> SSVEKKPEGVNTGAGDRHNLKTEWPELVGKSVEEAKKVILQDKPEAQIIVLPVGTIVTMEYRIDRVRLFVDKLDNIAEVPRV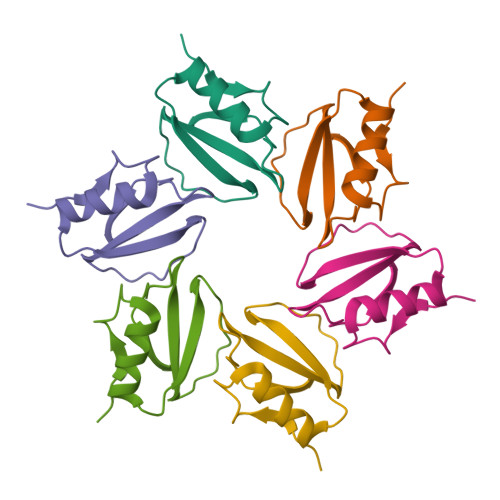G>[2x]MIFVKNLASVLSQEWSSTEKYPGVRWKFLIDADFDGSSGLSLGFAEIAPGGDLTLHYHSPAEIYVVTNGKGILNKSGKLETIKKGDVVYIAG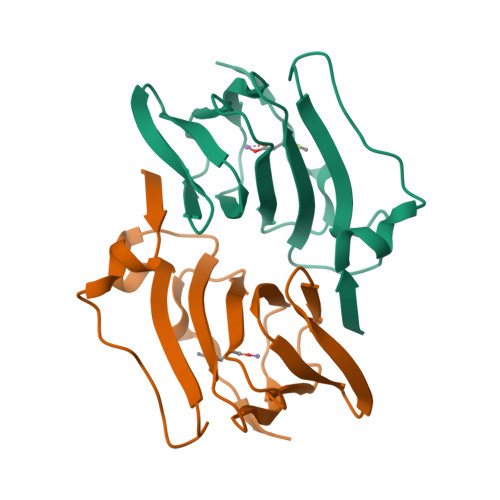NAEHALKNNGKETLEFYWIFPTDRFSEVEAFPAKQKSGHHHHHH> MTILKQMMRKLKNEKIHMTLIDPAAKSPDESAKIAKEAEMAGTDFIMVGGSTDIDERLMDQTVSAIKENTNLKVILFPGSSNMISRHADAIFFMSLLNSSDREFIVGHQVKASKFLSLLGIEKIPMAYLVFSPGMTVGRVGKANLIDSFDRETALSYSLAAQYMGFKLIYFEAGSGAPRPVSEDTISYVKSKINIPLIVGGGIRDPETAMRIALAGADMIVTGSIAE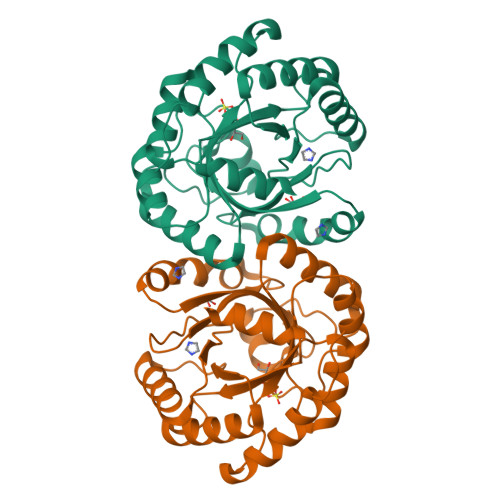KSNNVYSVLRNIIGKIKSIEIKNSV>[6x]MSAKSRTIGIIGAPFSKGQPRGGVEEGPTVLRKAGLLEKLKEQECDVKDYGDLPFADIPNDSPFQIVKNPRSVGKASEQLAGKVAEVKKNGRISLVLGGDHSLAIGSISGHARVHPDLGVIWVDAHTDINTPLTTTSGNLHGQPVSFLLKELKGKIPDVPGFSWVTPCISAKDIVYIGLRDVDPGEHYILKTLGIKYFSMTEVDRLGIGKVMEETLSYLLGRKKRPIHLSFDVDGLDPSFTPAT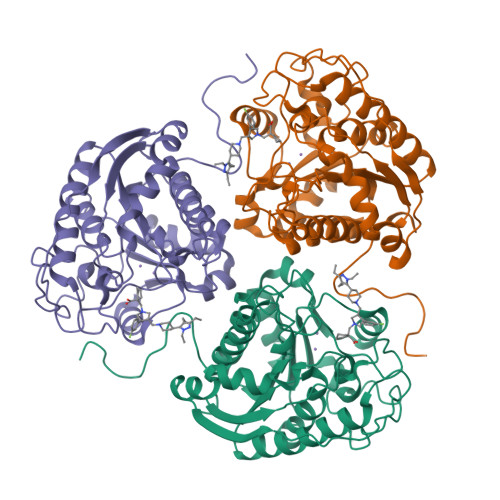GTPVVGGLTYREGLYITEEIYKTGLLSGLDIMEVNPSLGKTPEEVTRTVNTAVAITLACFGLAREGNHKPIDYLNPPK>[2x]MGSDKIHHHHHHENLYFQGMTNLGTAKNFWDATLYQDKHSFVWQYGEDLLQLLNPQPGEFILDLGCGTGQLTEKIAQSGAEVLGTDNAATMIEKARQNYPHLHFDVADARNFRVDKPLDAVFSNAMLHWVKEPEAAIASIHQALKSGGRFVAEFGGKGNIKYILEALYNALETLGIHNPQALNPWYFPSIGEYVNILEKQGFDVTYAALFNRPTTLA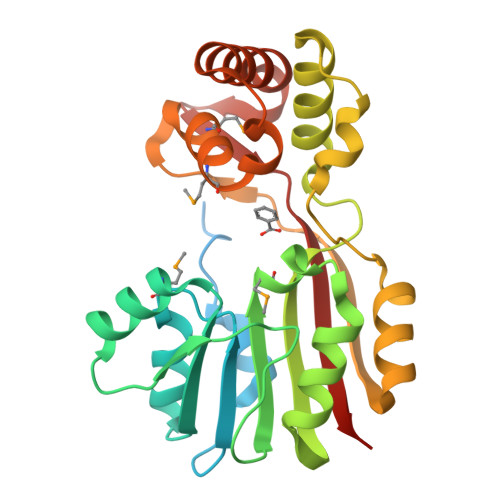EGEFGMANWIQMFASAFLVGLTPDQQVQLIRKVEATLQDKLYHQESWTADYRRIRIVSIKAQ> MAAPAAEAPLSHVQQALAELAKPKDDPTRKHVCVQVAPAVRVAIAETLGLAPGATTPKQLAEGLRRLGFDEVFDTLFGADLTIMEEGSELLHRLTEHLEAHPHSDEPLPMFTSCCPGWIAMLEKSYPDLIPYVSSCKSPQMMLAAMVKSYLAEKKGIAPKDMVMVSIMPCTRKQSEADRDWFCVDADPTLRQLDHVITTVELG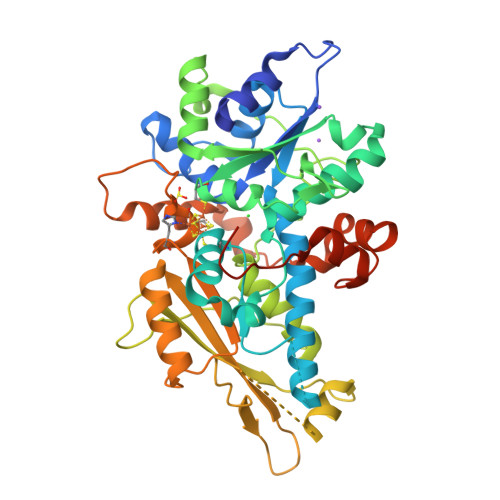NIFKERGINLAELPEGEWDNPMGVGSGAGVLFGTTGGVMEAALRTAYELFTGTPLPRLSLSEVRGMDGIKETNITMVPAPGSKFEELLKHRAAARAEAAAHGTPGPLAWDGGAGFTSEDGRGGITLRVAVANGLGNAKKLITKMQAGEAKYDFVEIMAHPAGCVGGGGQPRSTDKAITQKRQAALYNLDEKSTLRRSHENPSIRELYDTYLGEPLGHKAHELLHTHYVAGGVEEKDEKKSAWSHPQFEK> MQTNVPKFTAVAEQVSAVLSQYGITGPNRAIYQGFGLKVARALNRLGGGPALVNMINGLKAYYISAFN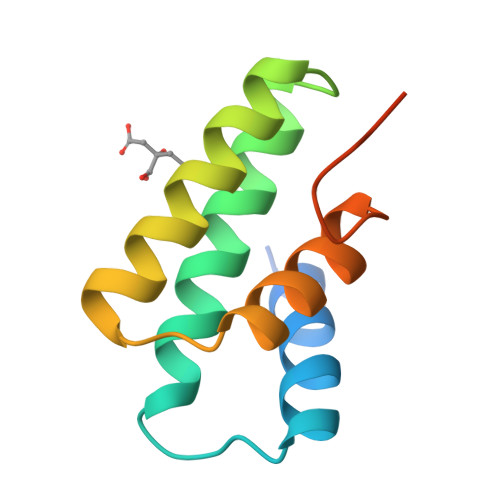ANPTVLDAVTDIITGSPTGYVSGGSGHHHHHH> P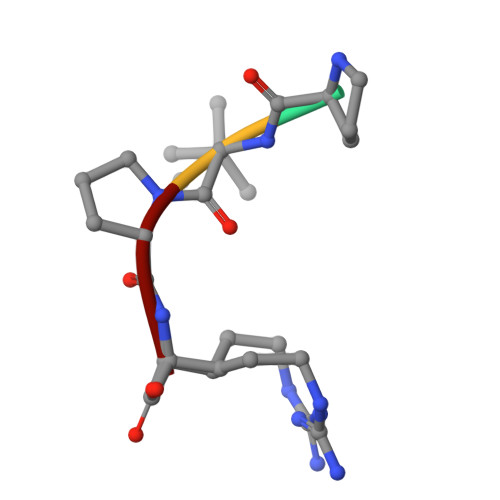VPR> 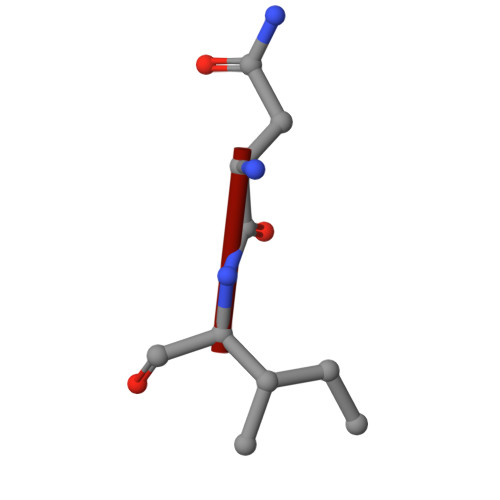DGMNLNI>[2x]Y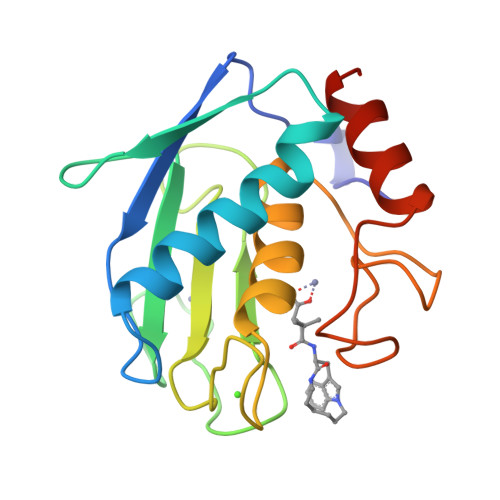SLFPNSPKWTSKVVTYRIVSYTRDLPHITVDRLVSKALNMWGKEIPLHFRKVVWGTADIMIGFARGAHGDSYPFDGPGNTLAHAFAPGTGLGGDAHFDEDERWTDGSSLGINFLYAATHELGHSLGMGHSSDPNAVMYPTYGNGDPQNFKLSQDDIKGIQKLYGKRSNS>MLVMNTPNGNSLSAAELTCGMIMCLARQIPQATASMKDGKWERKKFMGTELNGKTLGILGLGRIGREVATRMQSFGMKTIGYDPIISPEVSASFGVQQLPLEEIWPLCDFITVHTPLLPSTTGLLNDNTFAQCKKGVRVVNCARGGIVDEGALLRALQSGQCAGAALDVFTEEPPRDRALVDHENV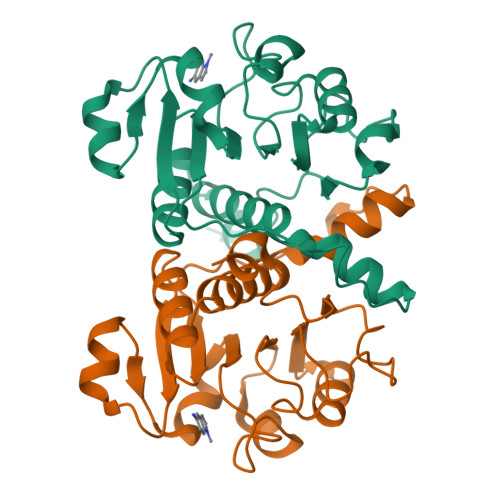ISCPHLGASTKEAQSRCGEEIAVQFVDMVKGKSLTGV[2x]>MTTLFKKYGPAVVMGVLSIALPQIALAAGTDTGESTATSIQTWLSTWIPIGCAIAIMVSCFMWMLHVIPASFIPRIVISLIGIGSASYLVSLTG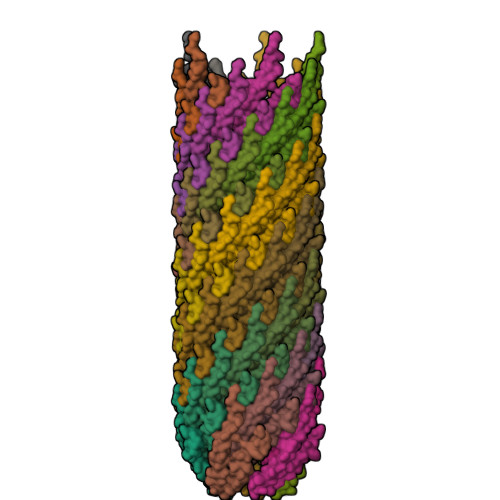VGS[70x]>[3x]GSHMPDWRQFCELHAQAAAVDFAHKFCRFLRDNPAYDT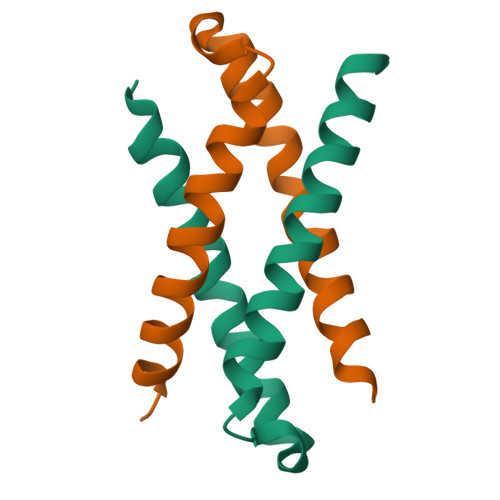PDAGASFSRHFAANFLDVFGEEVRRVLVAGP> LSKYGGECSKEHNTCTYRKDGKDHIVKCPSADNKKC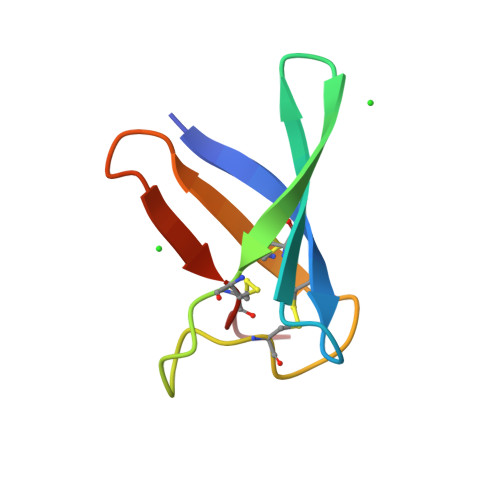KTDRHHCEYDDHHKTVDCDFRK>[2x]SQKFDVVVIGAGPGGYVAAIRAAQLGLKTACIEKYIGKEGKVALGGTCLNVGCIPSKALLDSSYKYHEAKEAFKVHGIEAKGVTIDVPAMVARKANIVKNLTGGIATLFKANGVTSFEGHGKLLANKQVEVTGLDGKTQVLEAENVIIASGSRPVEIPPAPLSDDIIVDSTGALEFQAVPKKLGVIGAGVIGLELGSVWARLGAEVTVLEALDKFLPAADEQIAKEALKVLTKQGLNIRLGARVT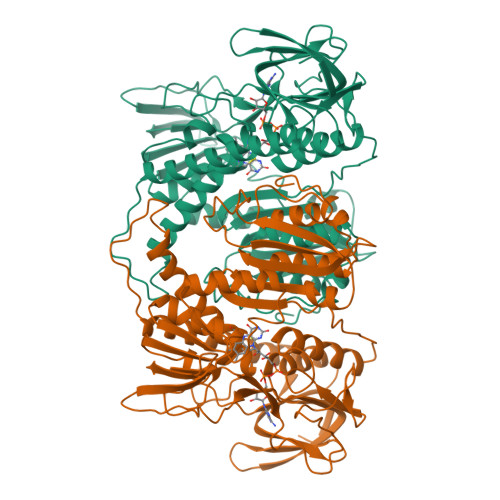ASEVKKKQVTVTFTDANGEQKETFDKLIVAVGRRPVTTDLLAADSGVTLDERGFIYVDDHCKTSVPGVFAIGDVVRGAMLAHKASEEGVMVAERIAGHKAQMNYDLIPSVIYTHPEIAWVGKTEQTLKAEGVEVNVGTFPFAASGRAMAANDTTGLVKVIADAKTDRVLGVHVIGPSAAELVQQGAIGMEFGTSAEDLGMMVFSHPTLSEALHEAALAVNGHAIHIANRKKR DExD/H-box RNA helicases, from virus and bacteria to eukaryotes, play important roles in processes including ribosome biogenesis, RNA processing and folding, ribonucleoprotein (RNP) remodeling, RNA nuclear export, the regulation of RNA translation and transcription, and nonsense-mediated RNA decay. DExD/H-box proteins often contain accessory regulatory domains and localization modules, but their cores consist of two RecA-like domains joined by a short flexible linker. The N-terminal domain is commonly referred to as conserved domain-1, or DEAD-domain, and the C-terminal domain as conserved domain-2, or helicase domain. Both domains contribute to the binding site for RNA substrates and both contribute to ATP hydrolysis. We used X-ray crystallography to determine the structures of the DEAD-domains of DDX2A, DDX2B, DDX5, DDX10, DDX18, DDX20, DDX47, DDX52, and DDX53, as well as the helicase domains of DDX25 and DDX41.

DDX25 (GRTH) is a testis specific, gonadotropin and androgen regulated protein that is essential for completion of spermatogenesis. The two helicase domains have a sequence identity of 23% and their structures superimpose with an r.m.s.d. of 3 Å. The helicase domain contributes to nucleotide coordination via motifs V and VI. A superposition of DDX19 with the DDX25 and DDX41 helicase domains shows that in the latter two structures part of motif VI is not visible in the electron density, indicating its flexibility. The conserved motifs IV and VI superpose well, whereas motif V shows different conformations in all three structures. In the free helicase domain structures motif V, an important RNA backbone interaction site is in a binding incompetent conformation.

>SMLTLNNIRQYYVLCEHRKDKYQALCNIYGSITIGQAIIFCQTRRNAKWLTVEMIQDGHQVSLLSGELTVEQRASIIQRFRDGKEKVLITTNVCARGIDVKQVTIVVNFDLPVKQGEEPDYETYLHRIGRTGRFGKKGLAFNMIEVDELPSLMKIQDHFNSSIKQLNAEDMDEIE[2x]> GHMIARGKFRSLTLINWNGFFARTFDFDELVTTLSGGNGAGKSTTMAGFVTALIPDLTLLNFRNTTEAGSTSSSRDKGLYGKLKAGVCYAVLETVNSRAQRIITGVRLQQIAGRDKKVDIRPFSLQNVPM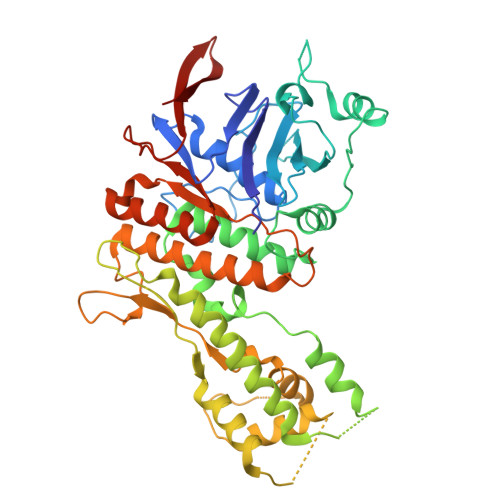TDSVISLFTEQVANKARVLSLNDLKEKFEETAVTFKPYHSITDYHSFMFDLGILPKRLRSSSDRNKFYKLIEASLYGGISSVITKSLRDYLLPENSGVRQAFQDMEAALRENSGGSGGSISAESVANILRKTIQREQNRILQLNQGLQNIAFGQVKGVRLVVNIRDTHSILLNALSDQHEQHKDLFESQKLSFSEALAMLYKRINPHIELGQRMPQTIGEELLDYRNYLDLEVETLRGAYGWMRAESSALSTGEAIGTGMSILLMVVQSWEEESRRMRAKDILPCRLLFLDQAARLDAMSINTLFELCERLDMQLLIAAPENISPERGTTYKLVRKILANQEYVHVVGLKGFG> GAMAEQQLRLPSPEVYRFVVKDSEENIVFEDNLQSRSGIPIIKGGTVVKLIERLTYHMYADPNFVRTFLTTYRSFCKPQELLSLLIERFEIPEPEPTDADKLAIEKGEQPISADLKRFRKEYVQPVQLRILNVFRHWVEHHFYDFERDLYLLERLESFISSVRGKAMKKWVESIAKIIRRKKQAQANGVSHNITFESPPPPIEWHISKPGHIETFDLMTLHPIEIARQLTLLESDLYRKVQPSELVGSVWTKEDKEINSPNLLKMIRHTTNLTLWFEKCIVEAENFEERVAVLSRIIEILQVFQDLNNFNGVLEIVSAVNSVSVYRLDHTFEALQERKRKILDEAV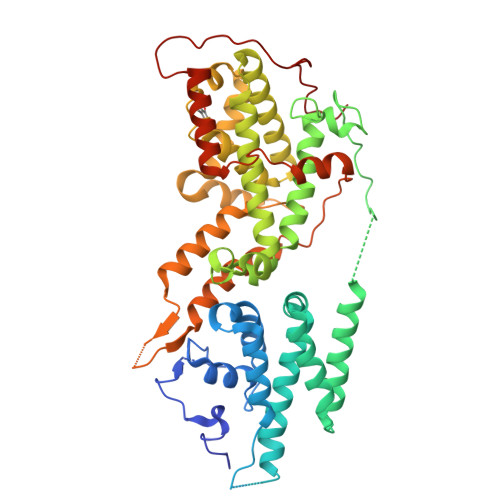ELSQDHFKKYLVKLKSINPPCVPFFGIYLTNILKTEEGNNDFLTRHGKDLINFSKRRKVAEITGEIQQYQNQPYCLRIEPDMRRFFENLNPMGSASEKEFTDYLFNKSLEIEPRNPKQPPRFPRKSTFSLKSPGIRPN> T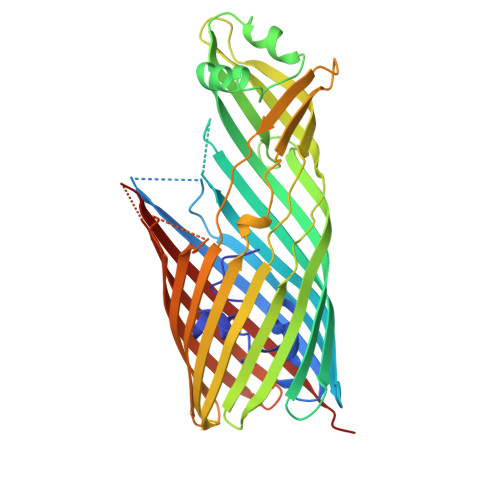DAFNLVGVGPVSQGMGGIGAAFNIGAQGMMLNPATLTQMQEGMHLGLGMDIITAELEVKNTATGEKADSHSRGRNNGPYVAPELSLVWRGERYALGVGAFASDGVGTQFGDTSFLSRTTTNNLNTGLENYSRLIVLRIPFSAAYQVNEKLSVGASLDAVWTSVNLGLLLDTTQIGTLVGQGQVSGSLMPALLSVPELSAGYLSADNHRASGGGVDSWGIGGRLGLTYQLTPKTRVGIVYNFKTHVGDLSGNADLTAVSAVAGNIPLSGELKLHNFEMPASLVAGISHEFSDQFAVAFDYKRVYWSDVMDDIEVNFKQKATGDTINLKLPFNYRDTNVYSLGAQYRYGANWVFRAGVHYAQLANPSSGTMPIIPSTPTTSLSGGFSYAFSPEDVVDFSLAYGFKKKVSNDSLPITDKPIEVSHSQIVTSISYTKSFHHHHHH>EDLHDKSELTDLALANAYGQYNHPFIKENIKSDEISGEKDLIFRNQGDSGNDLRVKFATADLAQKFKNKNVDIYGASFYYKCEKISENISECLYGGTTLNSEKLAQERVIGANVWVDGIQKETELIRTNKKNVTLQELDIKIRKILSDKYKIYYKDSEISKGLIEFDMKTPRDYSFDIYDLKGENDYEIDKIYEDNKTLKS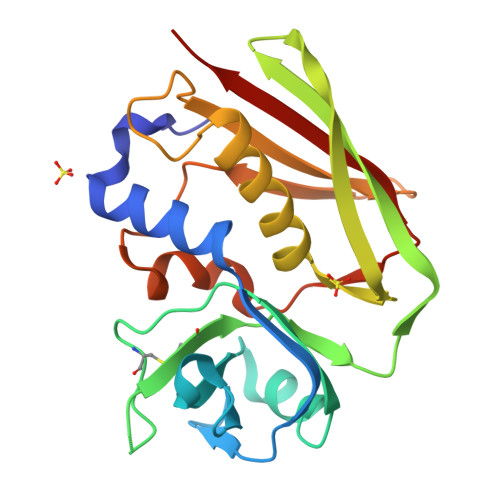DDISHIDVNLYTKKKV[2x]>GSKDQGGYGFAMRLKRRNWYPGAEESEVKLNESDWEATGLPTKPKELPKRQKSVIEKVETDGDSDIYSSPYLTPSNHQNGSAGNGVNQPKNQATGHENFQYVYSGWFYKHAASEKDFSNKKIKSGDDGYIFYHGEKPSRQLPASGKVIYKGVWHFVTDTKKGQDFREIIQPSKKQGDRYSGFSGDGSEEYSNKNESTLKDDHEGYGFTSNLEVDFGNKKLTGKLIRNNASLNNNTNNDKHTTQYYSLDAQITGNRFNGTATATDKKENETKLHPFVSDSSSLSGGFFGPQGEELGFRFLSDDQKVAVVGSAKTKDKLENGAAASGSTGAAASGGAAGTSSENSKLTTVLDAVELTLNDKKIKNLDNFSNAAQLVVDGIMIPLLPKDSESGNTQADKGKNGGTEFTRKFEHTPESDKKDAQAGTQTNGAQTASNTAGDTNGKTKTYEVEVCCSNLNYLKYGMLTRKNSKSAMQAGGNSSQADAKTEQVEQSMFLQGERTDEKEIPTDQNVVYRGSWYGHIANGTS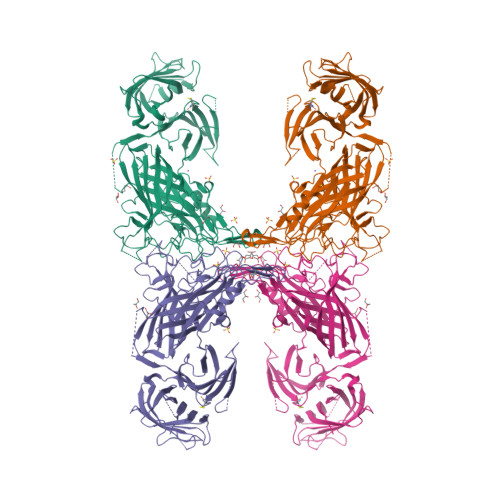WSGNASDKEGGNRAEFTVNFADKKITGKLTAENRQAQTFTIEGMIQGNGFEGTAKTAESGFDLDQKNTTRTPKAYITDAKVKGGFYGPKAEELGGWFAYPGDKQTEKATATSSDGNSASSATVVFGAKRQQPVQ[2x]>STCTFTSASEASESISSCSDVVLSSIEVPAGETLDLSDAADGSTITFEGTTSFGYKEWKGPLIRFGGKDLTVTMADGAVIDGDGSRWWDSKGTNGGKTKPKFMYIHDVEDSTFKGINIKNTPVQAISVQATNVHLNDFTIDNSDGDDNGGHNTDGFD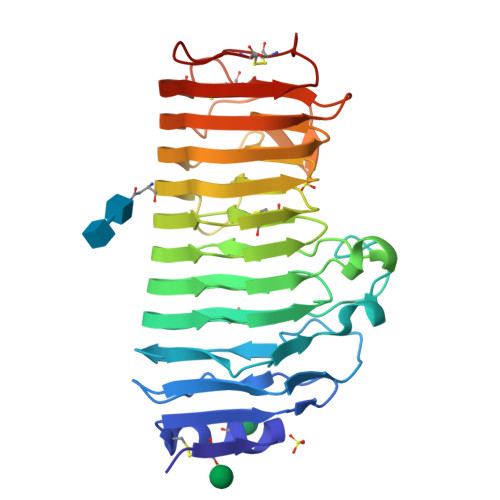ISESTGVYISGATVKNQDDCIAINSGESISFTGGTCSGGHGLSIGSVGGRDDNTVKNVTISDSTVSNSANGVRIKTIYKETGDVSEITYSNIQLSGITDYGIVIEQDYENGSPTGTPSTGIPITDVTVDGVTGTLEDDATQVYILCGDGSCSDWTWSGVDLSGGKTSDKCENVPSGASC[6x]>MGSSHHHHHHSSGRENLYFQGHMKNDTAALAADIVDFWKKAGPDKWFDKDAAFDNHFHDRFRDAHFAAARRELDGWLEGAESSLALMLLLDQFPRNCFRGTAHMYATDPLARFFADEAIRRGHDQAVSEDLRVFFYLPFSHAEDIAAQQRACD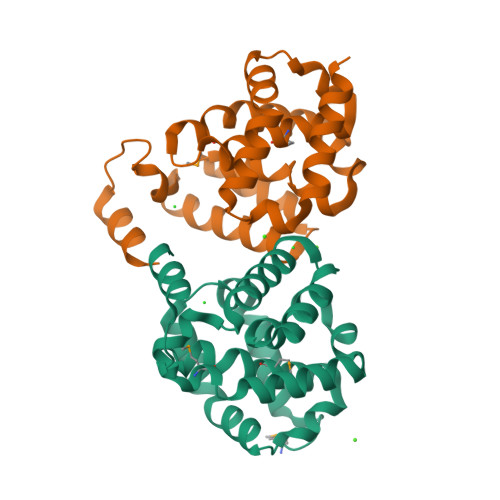LNQPLGGLYLHHAEEHRDIVERFGRFPHRNGILLRETTPEERQYLEEGGFSGGS[2x]>[2x]GHMSNTSWRKSEVLAVPLQPTLQQEVILARMEQILASRALTDDERAQLLYERGVLYDSLGLRALARNDFSQALAIRPDMPEVFNYLGIYLTQAGNFDAAYEAFDSVLELDPTYNYAHLNRGIALYYGGRDKLAQDDLLAFYQDDPNDPFRSLWLYLAEQKLDEKQAKEVLKQHFEKSDKEQWGWNIVEFYLGNISEQTLMERLKADATDNTSLAEHLSETNFYLGKYYLSLGDLDSATALFKLAVANNVHNFVEHRYALLELSLLGQDQDDLAESDQQ;>MNMFFRLTALAGLLAIAGQTFAVEDITRADQIPVLKEETQHATVSERVTSRFTRSHYRQFDLDQAFSAKIFDRYLNLLDYSHNVLLASDVEQFAKKKTELGDELRSGKLDVFYDLYNLAQKRRFERYQYALSVLEKPMDFTGNDTYNLDRSKAPWPKNEAELNALWDSKVKFDELSLKLTGKTDKEIRETLTRRYKFAIRRLAQTNSEDVFSLAMT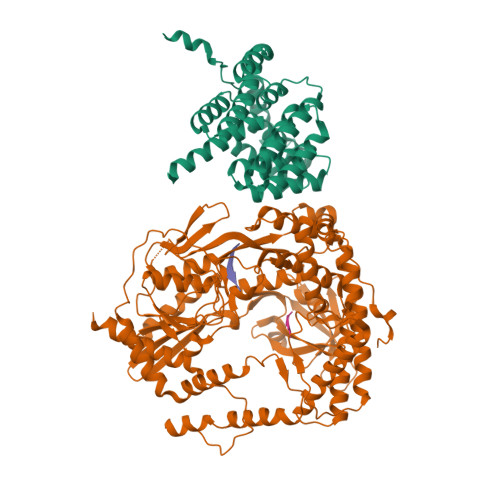AFAREIDPHTNYLSPRNTEQFNTEMSLSLEGIGAVLQMDDDYTVINSMVAGGPAAKSKAISVGDKIVGVGQTGKPMVDVIGWRLDDVVALIKGPKGSKVRLEILPAGKGTKTRTVTLTRERIRLEDRAVKMSVKTVGKEKVGVLDIPGFYVGLTDDVKVQLQKLEKQNVSSVIIDLRSNGGGALTEAVSLSGLFIPAGPIVQVRDNNGKVREDSDTDGQVFYKGPLVVLVDRFSASASEIFAAAMQDYGRALVVGEPTFGAGTVQQYRSLNRIYDQMLRPEWPALGSVQYTIQKFYRVNGGSTQRKGVTPDIIMPTGNEETETGEKFEDNALPWDSIDAATYVKSGDLTAFEPELLKEHNARIAKDPEFQNIMKDIARFNAMKDKRNIVSLNYAVREKENNEDDATRLARLNERFKREGKPELKKLDDLPKDYQEPDPYLDETVNIALDLAKLEKARPAEQPAPVK[2x];> AAAA;>[2x]AAAAAA;> LSRS>[4x]MAPKRSSDLFSQVVNSGPGSFLARQLGVPQPETLRRYRAGEPPLTGSLLIGGAGRVVEPLRAALEKDYDLVGNNLGGRWADSFGGLVFDATGITEPAGLKGLHEFFTPVLRNLGRCGRVVVVGGTPEAAASTNERIAQRA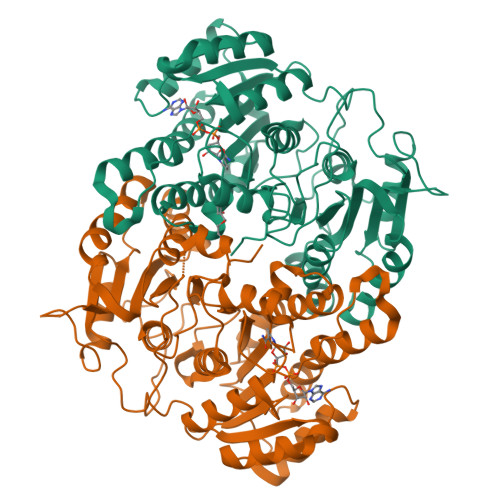LEGFTRSLGKELRRGATTALVYLSPDAKPAATGLESTMRFLLSAKSAYVDGQVFSVGADDSTPPADWEKPLDGKVAIVTGAARGIGATIAEVFARDGAHVVAIDVESAAENLAETASKVGGTALWLDVTADDAVDKISEHLRDHHGGKADILVNNAGITRDKLLANMDDARWDAVLAVNLLAPLRLTEGLVGNGSIGEGGRVIGLSSIAGIAGNRGQTNYATTKAGMIGITQALAPGLAAKGITINAVAPGFIETQMTAAIPLATREVGRRLNSLLQGGQPVDVAEAIAYFASPASNAVTGNVIRVCGQAMIGA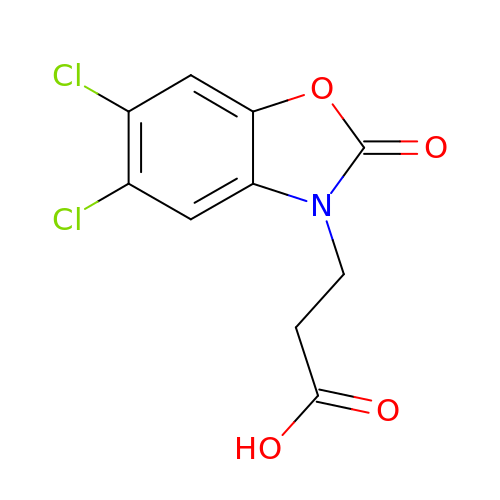3-(5,6-DICHLORO-2-OXOBENZO[D]OXAZOL-3(2H)-YL)PROPANOIC ACID | C10 H7 Cl2 N O4 | MIGAKMWKMLYGJX-UHFFFAOYSA-N> VMAEKSNKLDHI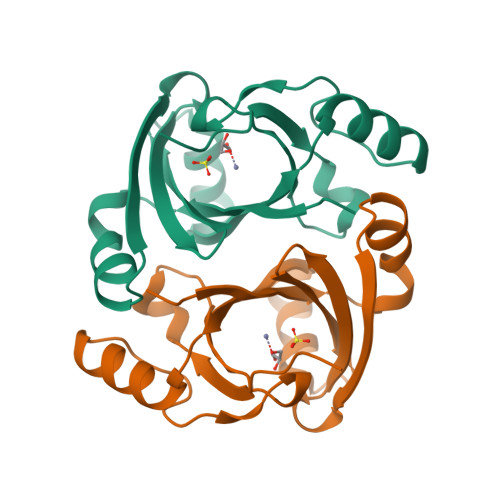GIAVTSIKDVLPFYVGSLKLKLLGMEDLPSQGVKIAFLEIGESKIELLEPLSEESPIAKFIQKRGEGIHHIAIGVKSIEERIQEVKENGVQMINDEPVPGARGAQVAFLHPRSARGVLYEFCEKKEQAENLYFQSHHHHHHWSHPQFEK2-{4-[(3S)-piperidin-3-yl]phenyl}-2H-indazole-7-carboxamide | C19 H20 N4 O | 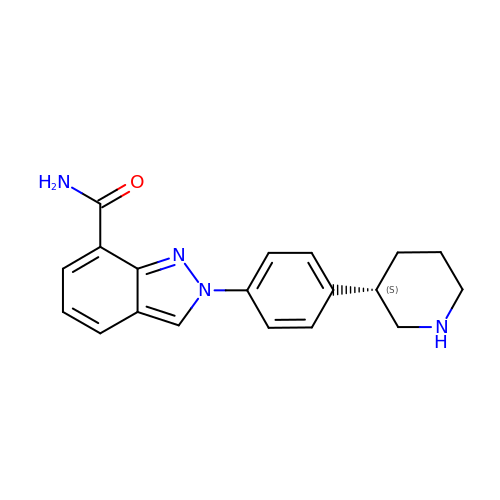PCHKPVIQAHNQLW-CQSZACIVSA-N Three capsid types have been recognized from the nuclei of herpesvirus-infected cells: empty A-capsids, scaffolding-containing B-capsids, and DNA-filled C-capsids. A unique portal vertex exists at a 12th I5 vertex through which the genome is translocated during assembly. Here, portal proteins assemble into a dodecameric basket-like structure that is thought to seed the assembly of scaffolding proteins, in turn driving the formation of spherical procapsids composed of MCP, SCP, and triplexes. A separate protein complex, the terminase, associates with the dodecameric portal and initiates genome packaging and the concurrent autoproteolytic cleavage of the scaffold.

Ten of the 12 monomers from the basket are linked to the turret helices, each of which consists of one long helix extending toward the portal cap and connecting to two smaller helices arranged in a small helical bundle. The two non-contributing portal monomers are presumably disordered or flexible beginning at their turret sequences. In C-capsids, D-capsids, and virions, the turret helices are fully extended, whereas in A- and B-capsids, they are retracted and positioned ~65 Å lower (Fig. 1F through J). C-capsid portal baskets are positioned higher at the portal vertex compared to their A- and B-capsid counterparts, which has been attributed to the densely packed genome pushing the portal up against the capsid shell. Only C-capsids ultimately become infectious virions.

>[10x]MTAPRSWAPTTRARGDTEALCSPEDGWVKVHPTPGTMLFREILHGQLGYTEGQGVYNVVRSSEATTRQLQAAIFHALLNATTYRDLEADWLGHVAARGLQPQRLVRRYRNAREADIAGVAERVFDTWRNTLRTTLLDFAHGLVACFAPGGPSGPSSFPKYIDWLTCLGLVPILRKRQEGGVTQGLRAFLKQHPLTRQLATVAEAAERAGPGFFELALAFDSTRVADYDRVYIYYNHRRGDWLVRDPISGQRGECLVLWPPLWTGDRLVFDSPVQRLFPEIVACHSLREHAHVCRLRNTASVKVLLGRKSDSERGVAGAARVVNKVLGEDDETKAGSAASRLVRLIINMKGMRHVGDINDTVRSYLDEAGGHLIDAPAVDGTLPGFGKGGNSRGSAGQDQGGRAPQLRQAFRTAVVNNINGVLEGYINNLFGTIERLRETNAGLATQLQERDRELRRATAGALERQQRAADLAAESVTGGCGSRPAGADLLRADYDIIDVSKSMDDDTYVANSFQHPYIPSYAQDLERLSRLWEHELVRCFKILCHRNNQGQETSISYSSGAIAAFVAPYFESVLRAPRVGAPITGSDVILGEEELWDAVFKKTRLQTYLTDIAALFVADVQHAALPPPPSPVGADFRPGASPRGRSRSRSPGRTAPGAPDQGGGIGHRDGRRDGRR> LSEEQQHIIAILLDAHHKTYDPTYADFRDFRPPVRMDGSTGSVTLDLSPLSMLPHLADLVSYSIQKVIGFAKMIPGFRDLTSDDQIVLLKSSAIEVIMLRSNQSFTMDDMSWDCGSQDYKYDVTDVSKAGHTLELIEPLIKFQVGLKKLNLHEEEHVLLMAICIVSPDRPGVQDAKLVEAIQDRLSNTLQTYIRCRHPPPGSHQLYAKMIQKLADLRSLNEEHSKQYRSLSFQPENSM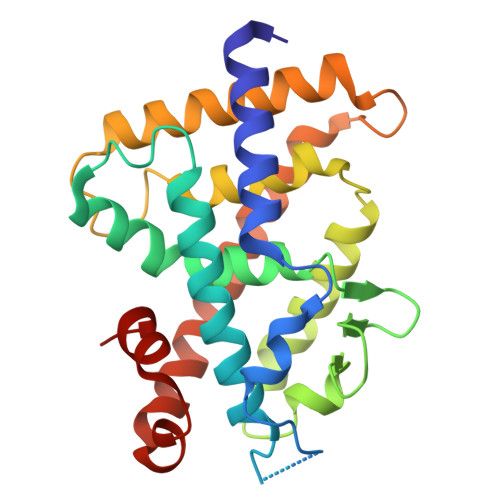KLTPLVLEVFGN> INITSSASQEGTRLNLICTVWHKKEEAEGFVVFLCKDRSGDCSPETSLKQLRLKRDPGIDGVGEISSQLMFTISQVTPLHSGTYQCCARSQKSGIRLQGHFFSILFTETG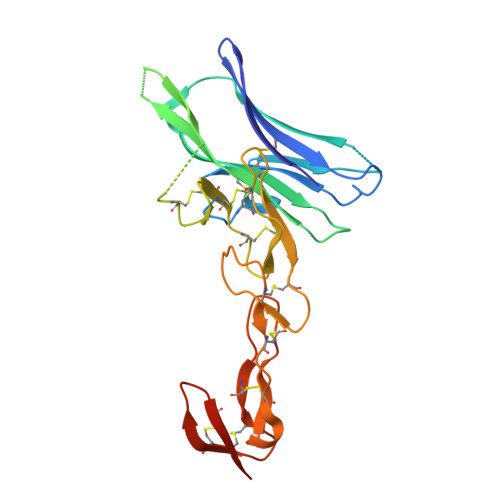NYTVTGLKGGGGSGGGGSGGGGSGGGGSLPSCKEDEYPVGSECCPKCSPGYRVKEACGELTGTVCEPCPPGTYIAHLNGLSKCLQCQMCDPAMGLRASRNCSRTENAVCGCSPGHFCIVQDGDHCAACRAYATGHHHHHH> SNAMLSPEALTTAVDAAQQAIALADTLDVLARVKTEHLGDRSPLALARQALAVLPKEQRAEAGKRVNAARNAAQRSYDERLATLRAERDAAVLVAEGIDVT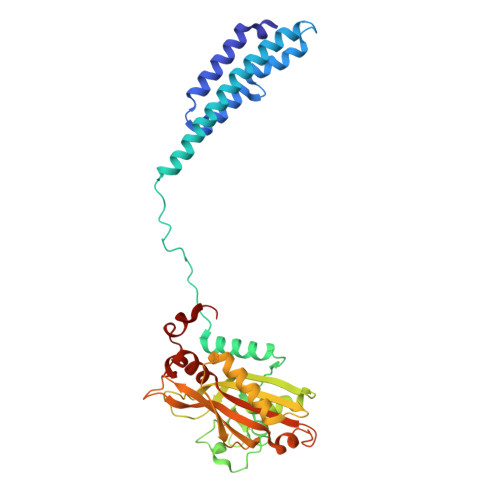LPSTRVPAGARHPIIMLAEHVADTFIAMGWELAEGPEVETEQFNFDALNFPADHPARGEQDTFYIAPEDSRQLLRTHTSPVQIRTLLARELPVYIISIGRTFRTDELDATHTPIFHQVEGLAVDRGLSMAHLRGTLDAFARAEFGPSARTRIRPHFFPFTEPSAEVDVWFANKIGGAAWVEWGGCGMVHPNVLRATGIDPDLYSGFAFGMGLERTLQFRNGIPDMRDMVEGDVRFSLPFGVGA> GAMEPTMDLSAFKDGLEVIVPNPITTLVPSTGYPRPTATWCFGDKVLETGDRVKMKTLSAYAELVISPSERSDKGIYTLKLENRVKTISGEIDVNVIARPSAPKELKFGDITKDSVHLTWEPPDDDGGSPLTGYVVEKREVSRKTWTKVMDFVTDLEFTVPDLVQGKEY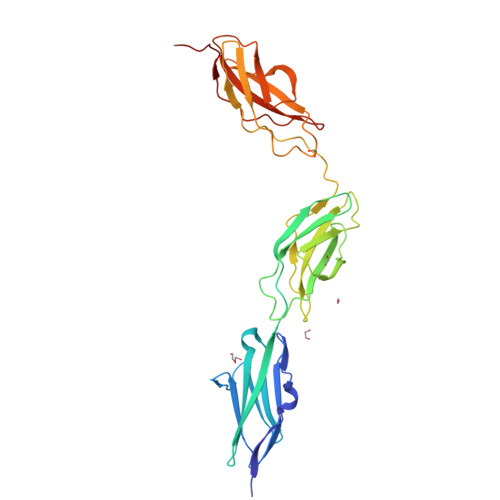LFRVCARNKCGPGEPAYVDEPVNMSTPATVPDPPENVKWRDRTANSIFLTWDPPKNDGGSRIKGYIVERCPRGSDKWVACGEPVAETKMEVTGLEEGKWYAYRVKALNRQGASKPSRPTEEIQAVDTQEAP> AMEPQVTLNVTFKNEIQSFLVSDPENTTWADIEAMVKVSFDLNTIQIKYLDEEN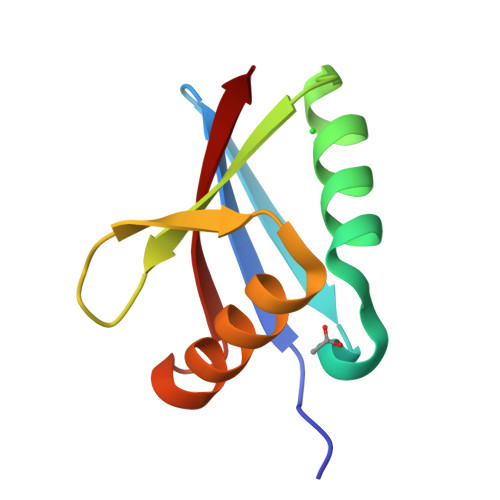EEVSINSQGEYEEALKMAVKQGNQLQMQVHEG>[2x]NDVARGIVKADVAQNNFGLYGQGQIVAVADTGLDTGRNDSSMHEAFRGKITALYALGRTNNANDPNGHGTHVAGSVLGNATNKGMAPQANLVFQSIMDSGGGLGGLPANLQTLFSQAYSAGARIHTNSWGAPVNGAYTTDSRNVDDYVRKNDMTILFAAGNEGPGSGTISAPGTAKNAITVGATENLRPSFGSYADNIN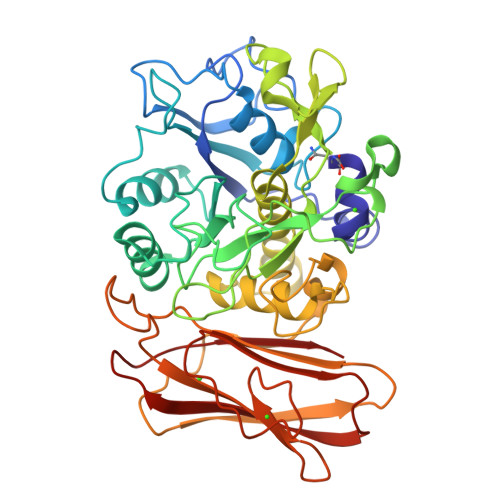HVAQFSSRGPTRDGRIKPDVMAPGTYILSARSSLAPDSSFWANHDSKYAYMGGTSMATPIVAGNVAQLREHFVKNRGVTPKPSLLKAALIAGAADVGLGFPNGNQGWGRVTLDKSLNVAFVNETSPLSTSQKATYSFTAQAGKPLKISLVWSDAPGSTTASLTLVNDLDLVITAPNGTKYVGNDFTAPYDNNWDGRNNVENVFINAPQSGTYTVEVQAYNVPVGPQTFSLAIVH> MRGSHHHHHHGLVPRGSMIRTMLQGKLHRVKVTHADLHYEG;> XCAIDQDFLDAAGILENEAIDIWNVTNGKRFSTYAIAAERGSRIISVQGAAAHCASVGDIVIIASFVTMPDEEARTWRPN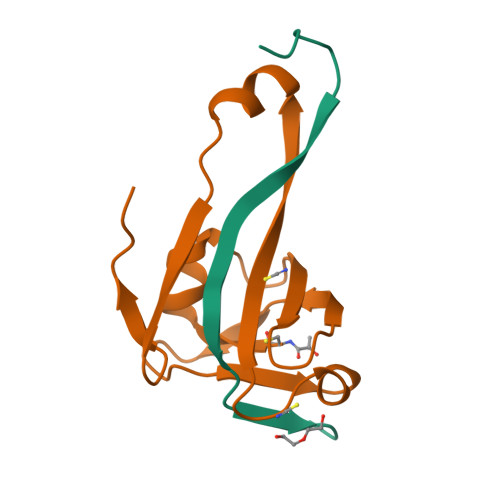VAYFEGDNEMKRTAK>SHMLFQNVSIAGLAHIDAPHTLTSKEINERLQPTY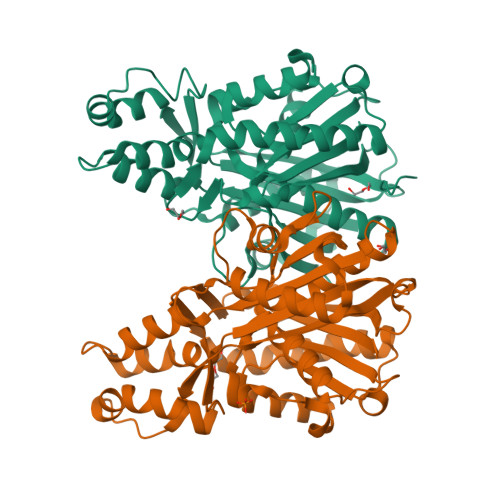DRLGIKTDVLGDVAGIHARRLWDQDVQASDAATQAARKALIDANIGIEKIGLLINTSVSRDYLEPSTASIVSGNLGVSDHCMTFDVANASLAFINGMDIAARMLERGEIDYALVVDGETANLVYEKTLERMTSPDVTEEEFRNELAALTLGCGAAAMVMARSELVPDAPRYKGGVTRSATEWNKLCRGNLDRMVTDTRLLLIEGIKLAQKTFVAAKQVLGWAVEELDQFVIHQVSRPHTAAFVKSFGIDPAKVMTIFGEHGNIGPASVPIVLSKLKELGRLKKGDRIALLGIGSGLNCSMAEVVW[2x]>[8x]MGSSHHHHHHSQDPMLNSFKLSLQYILPKL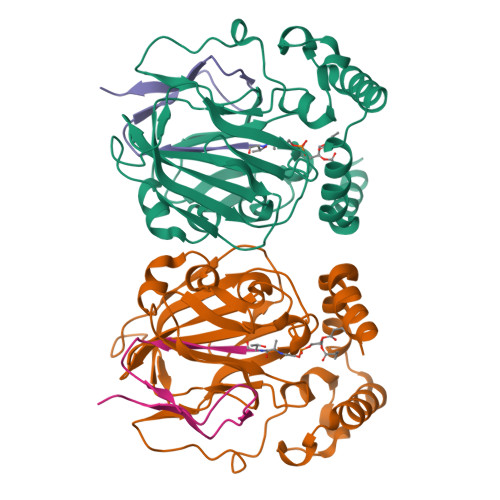WLTRLAGWGASKRAGWLTKLVIDLFVKYYKVDMKEAQKPDTASYRTFNEFFVRPLRDEVRPIDTDPNVLVMPADGVISQLGKIEEDKILQAKGHNYSLEALLAGNYLMADLFRNGTFVTTYLSPRDYHRVHMPCNGILREMIYVPGDLFSVNHLTAQNVPNLFARNERVICLFDTEFGPMAQILVGATIVGSIETVWAGTITPPREGIIKRWTWPAGENDGSVALLKGQEMGRFKLG;>[8x]XTVINLFAPGKVNLVEQLESLSVTKIGQPLAVSTET>[2x]MDTKLLDILACPICKGPLKLSADKTELISKGAGLAYPIRDGIPVMLESEARTLT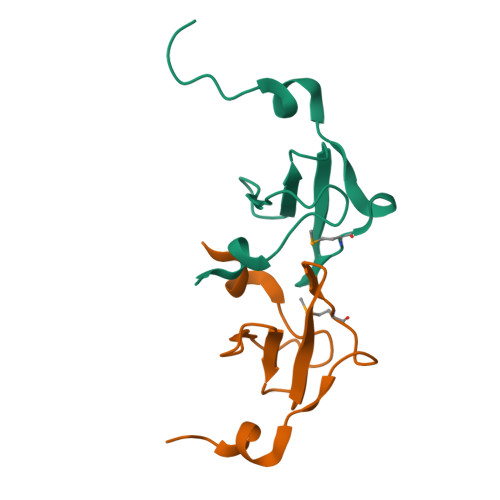TEERLDKLEHHHHHH As a part of efforts to develop new therapeutics and diagnostics for melioidosis, the Seattle Structural Genomics Center for Infectious Disease (SSGCID) has determined the crystal structure of betaine aldehyde dehydrogenase (BADH) from B. pseudomallei (BpBADH). BADH catalyzes the irreversible oxidation of betaine aldehyde to the osmoprotectant betaine and is being investigated as a drug target for drug-resistant bacteria, notably Pseudomonas aeruginosa, because its inhibition blocks choline catabolism and leads to the accumulation of the highly toxic betaine aldehyde. The structure also contains 21 helices, 21 strands, four β-hairpins, four β-bulges and 25 helix–helix interactions. BpBADH has a prototypical BADH topology and shares considerable structure and sequence similarity with the ortholog from P. aeruginosa (PaBADH). The 489 amino acids in each monomer fold as 20.4% β-strand, 39.3% α-helix, 2.5% 310-helix and 37.8% loops, forming six β-α-β motifs that contain five β-sheets (four mixed and one antiparallel).

The monomers are very similar and have an r.m.s.d. of ∼0.17 Å for main-chain atoms.

> MSVYGLQRLYIAGAHADATSGKTFDTFDPATGELLARVQQASADDVDRAVASAREGQREWAAMTAMQRSRILRRAVELLRERNDALAELEMRDTGKPIAETRAVDIVTGADVIEYYAGLATAIEGLQVPLRPESFVYTRREPLGVCAGIGAWNYPIQIACWKSAPALAAGNAMIFKPSEVTPLSALKLAEIYTEAGVPAGVFNVVQGDGSVGALLSAHPGIAKVSFTGGVETGKKVMSLAGASSLKEVTMELGGKSPLIVFDDADLDRAADIAVTANFFSAGQVCTNGTRVFVQQAVKDAFVERVLARVARIRVGKPSDSDTNFGPLASAAQLDKVLGYIDSGKAEGAKLLAGGARLVNDHFASGQYVAPTVFGDCRDDMRIVREEIFGPVMSILSFETEDEAIARANATDYGLAAGVVTENLSRAHRAIHRLEAGICWINTWGESPAEMPVGGYKQSGVGRENGITTLEHYTRIKSVQVELGRYQPVFGHHHHHH>[2x]GSHMCAAQMPPLAHIFRGTFVHSTWTCPMEVLRDHLLGVSDSGKIVFLEEASQQEKLAKEWCFKPCEIRELSHHEFFMPGLVDTHIHASQYSFAGSSIDLPLLEWLTKY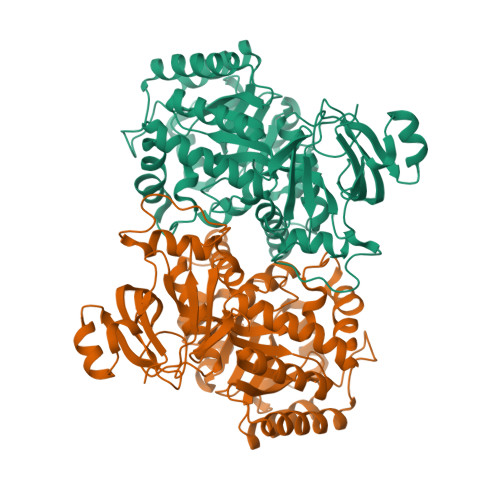TFPAEHRFQNIDFAEEVYTRVVRRTLKNGTTTACYFATIHTDSSLLLADITDKFGQRAFVGKVCMDLNDTFPEYKETTEESIKETERFVSEMLQKNYSRVKPIVTPGNGVSETLMGELGNIAKTRDLHIQSHISENRDEVEAVKNLYPSYKNYTSVYDKNNLLTNKTVMAHGCYLSAEELNVFHERGASIAHCPNSNLSLSSGFLNVLEVLKHEVKIGLGTDVAGGYSYSMLDAIRRAVMVSNILLINKVNEKSLTLKEVFRLATLGGSQALGLDGEIGNFEVGKEFDAILINPKASDSPIDLFYGDFFGDISEAVIQKFLYLGDDRNIEEVYVGGKQVVPFSSSV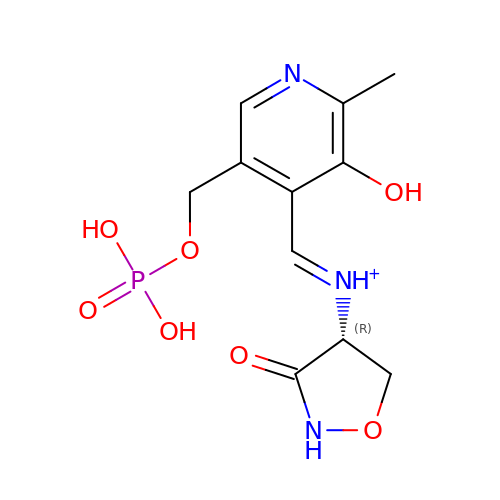(~{E})-[2-methyl-3-oxidanyl-5-(phosphonooxymethyl)pyridin-4-yl]methylidene-[(4~{R})-3-oxidanylidene-1,2-oxazolidin-4-yl]azanium | C11 H15 N3 O7 P | PWALIMMCDFLLIJ-RZTFRGLUSA-O> AKKRVFTFGKGRSEGNKDMKSLLGGKGANLAEMASIGLSVPPGLTISTEACEEYQQNGKKLPPGLWDEILEGLRYVQKEMSASLGDPSKPLLLSVRSGAAISMPGMMDTVLNLGLNDEVVAGLAGKSGARFAYDSYRRFLDMFGNVVMGIPHSLFDEKLEEMKAEKGVHLDTDLTAADLKDLVEQYKNVYVEAKGEKFPTDPKKQLELAVNAVFDSWDSPRANKYRSINQITGLKGTAVNIQCMVFGNMGNTSGTGVLFTRNPSTGEKKLYGEFLVNAQGEDVVAGIRTPEDLATMETCMPEAYRELVENCKILERHYKDMMDIEFTVQENRLWMLQCRTGKRTGKGAVRIAVDMVNEGLIDTRTAIKRVETQHLDQLLHPQFENPSAYKSHVVATGLPASPGAAVGQVVFSAEDAETWHAQGKSAILVRTETSPEDVGGMHAAAGILTARGGMTSHAAVVARGWGKCCVSGCADIRVNDDMKVLTIGDRVIKEGDWLSLNGSTGEVILGKQLLAPPAMSNDLETFMSWADQVRRLKVMANADTPNDALTARNNGAQGIGLCRTEHMFFASDERIKAVRKMIMAVTPEQRKAALDLLLPYQRSDFEGIFRAMDGLPVTIRLLDPPLHEFLPEGDLEHIVNELAVDTGMSEDEIYSKIEKLSEVNPMLGFRGCRLGISYPELTEMQVRAIFQAAVSMNNQGVTVIPEIMVPLVGTPQELRHQIGVIRGVAANVFAEMGLTMDYKVGTMIEIPRAALIAEEIAKEAEFFSFGTNDLTQMTFGYSRDDVGKFLQIYLSQGILQHDPFEVLDQKGVGQLIKMATEKGRAANPNLKVGICGEHGGEPSSVAFFDGVGLDYVSCSPFRVPIARLAAAQVVV

Here, the rate limiting regeneration of the primary CO2 acceptor phosphoenolpyruvate (PEP) is catalyzed by the multi-domain protein pyruvate phosphate dikinase (PPDK). Previous studies emphasize that PPDK has a modular structure consisting of distinct substrate binding domains for PEP/pyruvate at the C-terminus (PBD) and for nucleotides ATP/AMP at the N-terminus (NBD, aa 1–340). A central domain (CD, aa 380–515) catalyzing the phosphoryl group transfer from ATP to pyruvate–or from PEP to AMP–via a phospho-histidine intermediate mediates a catalytic cross-talk between the distant substrate binding domains. Distinct conformational states resolved in crystal structures from maize and the non-plant organisms Clostridium symbiosum and Trypanosoma brucei suggest that the phosphoryl group transfer in the catalytic cycle is accompanied by a large swiveling motion of the CD from a position next to the NBD to a position facing the PBD (~110° and 45 Å).

Hence, compared to the two extreme conformations of the CD next to the NBD or PBD previously resolved, the CD in the F. pringlei conformational intermediate shows about 50% of the rotational and translational movement of the proposed complete swiveling motion. Remarkably, in this structure the CD is positioned in an intermediate state between the NBD and PBD, thereby enlarging the solvent accessibility of the PEP binding pocket. The CD position is not enforced by crystal contacts and therefore represents a genuine structural intermediate of the proposed swiveling mechanism. The entire domain is rather mobile resulting in higher B-factors in this region. Concerning the substrate and cofactor binding site, density is visible for both ligands, PEP and 2'-Br-dAppNHp. Additional density in the conformational intermediate was observed in close proximity of the phosphoryl group of the PEP substrate. This additional density might reflect an alternative position of the PEP substrate in the PBD. To elucidate critical contacts mediating interactions between the CD or linker domain (LD) and the PBD, the FpPPDK conformational intermediate was analyzed with Cytoscape30 and RINalyzer31, which identified a salt bridge formed between E804 and R462, and non-polar patches at I864 in the PBD and L378 in the LD likely involved in hydrophobic interactions. Both interactions may restrict rotational freedom of the CD in this state, promoting the stepped motion of the CD. Third, we identify a stable conformational intermediate of the CD swivelling motion, revealed by pronounced minima in the PMFs at a distanceCD–PBD ~30–35 Å, which is structurally highly similar to the intermediate state IV found in the FpPPDK crystal structure (located at a distanceCD–PBD ~25 Å) as shown by a Cα atom RMSD of 2.7 Å.N-(2-hydroxyethyl)-N,N-dimethyl-3-sulfopropan-1-aminium 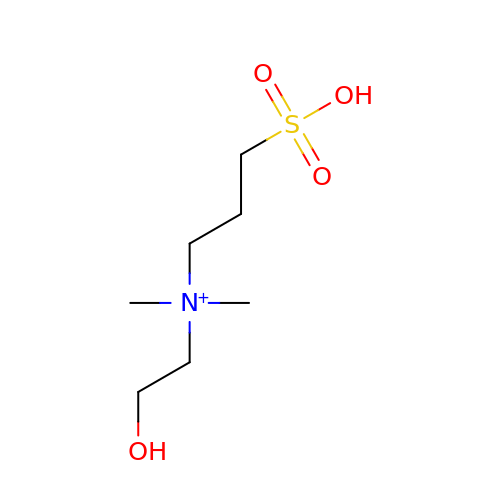| C7 H18 N O4 S | CNXPCGBLGHKAIL-UHFFFAOYSA-O> MRVTQK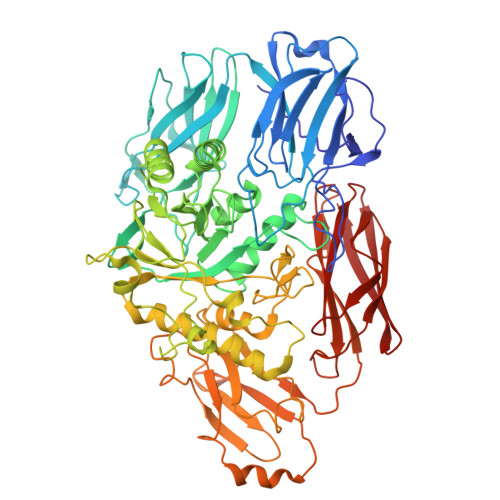LNHGWIFAEGAADPATPLAGETVTLPHNAVDLPLSYFDETSYQRAFTYQRVIAWDDAWQGRRVQLRFDGAMADNVVWVNGVQVVAHPDGYTPFVADLTDHLRPGDNLVTVRIDGSENPAIPPFGAQIDYLTYAGIYRDVWLMVLPERHLTNARILTPDALSDAKTVVIRPEVTAPGPVRARLLDGDREIAATEGEGELTLAGLTGLSLWSTDNPQLYTVELTLPDSGDVTTHRFGFRTAEWTPQGFLLNGQPMKLRGLNRHQSWAHQGYAAGRHAQERDAEIVRHDLCCNMVRTSHYPQSTWFLDRCDEIGLLVFEEIPGWQHIGDQAWQDRSVDNVRAMITRDWNHPSIVIWGVRINESPDNHDFYVRTNALARELDPTRAIGGVRCITDSEMLEDVYTMNDFILDESELPLINRPRTALRPTEEVTGIKKPVPYLVTEYNGHMFPTKAQDPELRQMEHVIRHLEVLNAAHGDPAISGCIGWCMFDYNTHKDFGAGDRICHHGVMDIWREPKFAAHAYGSQKPPSEGIVMEPVTFWARGERNIGGVLPLIVLTNCDEVEFECAGVTRRVGPDRERFPHLPRPPVIIDHRHISAEELGQWGMSWHPGRITGWLNGEQVALREYVADPLPTTLQIAPDRDTLPADGDIDLRVMLRALDQVGNRLPFLDAGIAVTVDGPARLIGPDLRMLQGGTTGMLLRLTGDAGTIRITARHPQFPEAVATVTVG>SQDASDGLQRLHMLQISYFRDPYHVWYQGNASLGGHLTHVLEGPDTNTTIIQLQPLQEPESWARTQSGLQSYLLQFHGLVRLVHQERTLAFPLTIRCFLGCELPPEGSRAHVFFEVAVNGSSFVSF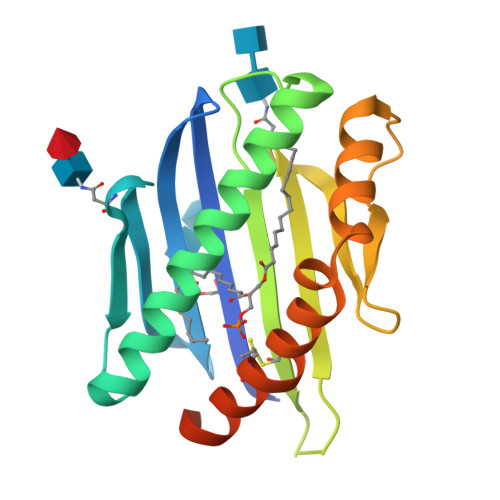RPERALWQADTQVTSGVVTFTLQQLNAYNRTRYELREFLEDTCVQYVQKHISAENTKGSQTSRSYTS[4x]> KKVDHRAPGAEEDDSELQRAWGALIKEKEQSR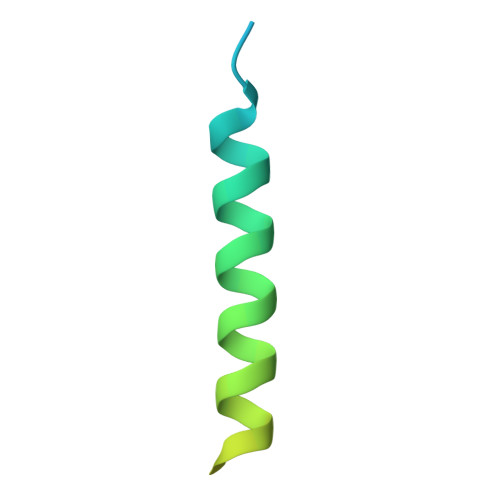QKKSRLDNLPSLQIEVSRESSSGSEAES>GEAPVQPILSSVPTTEVSTGVKFQVGDLVWSKVGTYPWWPCMVSSDPQLEVHTKINTRGAREYHVQFFSNQPERAWVHEKRVREYKGHKQYEELLAEATKQASNHSEKQKIRKPRPQRERAQWDIGIAHAEKALKMTREERIE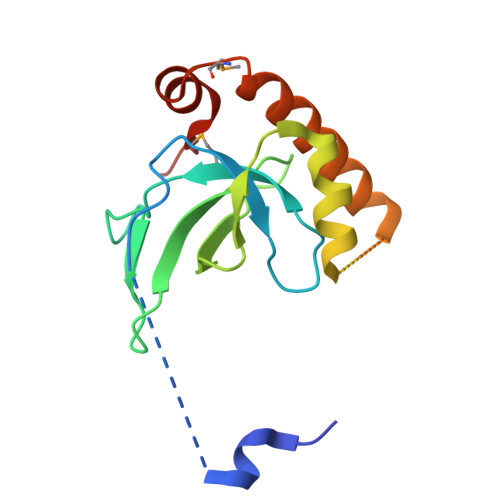QYTFIYIDKQ[4x]>HHHHHHMLENIRDAVRKFLTGSTPYEKAVDEFIKDLQKSLISSDVNVKLVFSLTAKIKERLNKEKPPSVLERKEWFISIVYDELSKLFGGDKEPNVNPTKLPFIIMLVGVQGSGKTTTAGKLAYFYKKRGYKVGLVAADVYRPAAYDQLLQLGNQIGVQVYGEPNNQNPIEIAKKGVDIFVKNKMDIIIVDTAGRHGYGEETKLLEEMKEMYDVLKPDDVILVIDASIGQKAYDLASRFH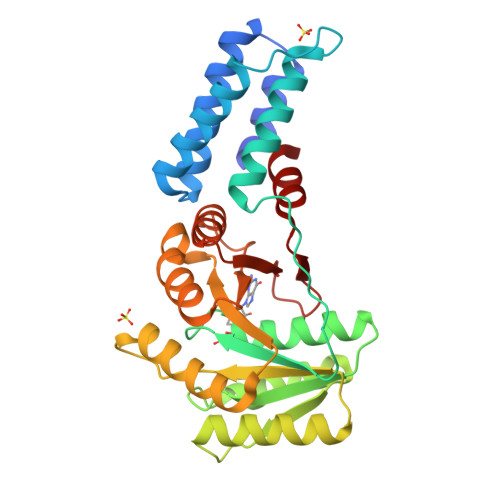QASPIGSVIITKMDGTAKGGGALSAVVATGATIKFIGTGEKIDELETFNAKRFVSRILG[2x]>[2x]GMRKGQETRERVVAQAAALFNVSGYAGTAISDIMAATGLEKGGIYRHFESKEQLALAAFDYAAEKVRERFA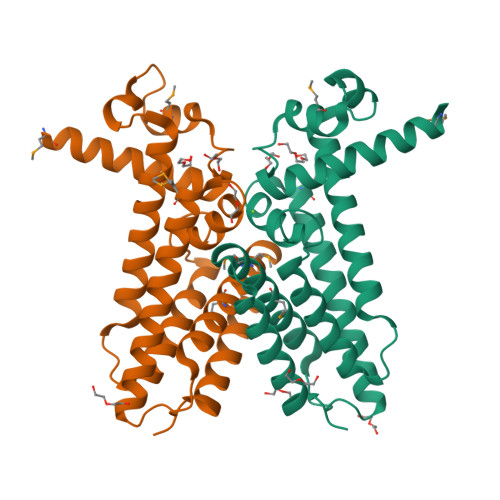VGLAGHKHTVDTIIAFLDVFRSYAERPPLVGGCPILNTAIESDDTNPMLRERVRAVIDEWRETIRTLVQTGIARGEIRPEVDADRLALLIIATMEGAVMLARILETATPLEHAYTHLATYITQQVRLA>[2x]MTEIATTSGARSVGLLSVGAYRPERVVTNDEICQHIDSSDEWIYTRTGIK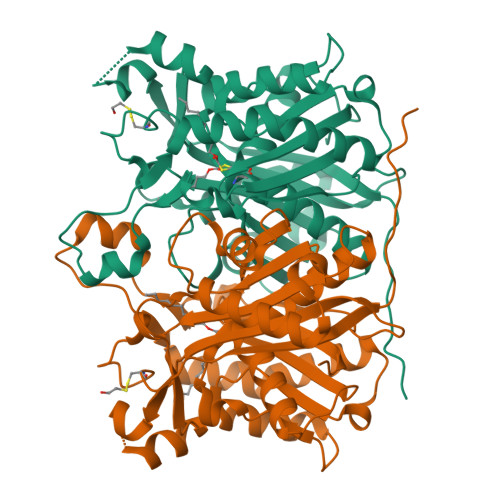TRRFAADDESAASMATEACRRALSNAGLSAADIDGVIVTTNTHFLQTPPAAPMVAASLGAKGILGFDLSAGCAGFGYALGAAADMIRGGGAATMLVVGTEKLSPTIDMYDRGNCFIFADGAAAVVVGETPFQGIGPTVAGSDGEQADAIRQDIDWITFAQNPSGPRPFVRLEGPAVFRWAAFKMGDVGRRAMDAAGVRPDQIDVFVPHQANSRINELLVKNLQLRPDAVVANDIEHTGNTSAASIPLAMAELLTTGAAKPGDLALLIGYGAGLSYAAQVVRMPKG8-[4-(1-ethyl-1,2,3-triazol-4-yl)butyl]-2,2-bis(fluoranyl)-4,6,10,12-tetramethyl-3-aza-1-azonia-2-boranuidatricyclo[7.3.0.0^{3,7}]dodeca-1(12),4,6,8,10-pentaene | C21 H28 B F2 N5 | 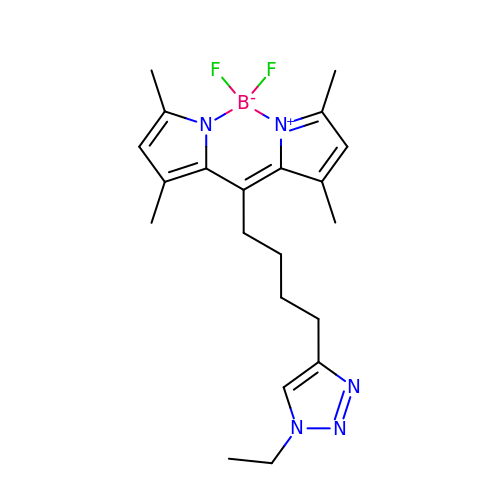SOYAGSBCXYKTSE-UHFFFAOYSA-N Galectins are multi-purpose effectors acting via interactions with distinct counterreceptors based on protein-glycan/protein recognition. We report here the first crystallographic information on the N-terminal extension of the carbohydrate recognition domain of rat galectin-5, which is precisely described as an N-tailed proto-type-like galectin. The overall fold in ligand-free and -loaded rGal-5 is composed of two antiparallel β-sheets (F1 to F5 and S1 to S6 strands) that form the characteristic β-sandwich structure. The presented data shows that the N-terminal extension can adopt an ordered structure and shapes the hypothesis that a ligand-induced shift in the equilibrium between flexible and ordered conformers potentially acts as a molecular switch, enabling new contacts in this region.

Our attempts to crystallize rGal-5 bound to the blood-group B tetrasaccharide were unsuccessful. Thus, we decided to test chicken GRIFIN (cGRIFIN) as a model for the binding of this compound. We were able to obtain crystals of cGRIFIN in the presence of the blood-group B tetrasaccharide. These crystals diffracted up to a resolution of 1.14 Å. The GalB moiety fully superposes with the galactose moiety of lactose, forming H-bonds with His46, Asn48, Arg50, Asn59 and Glu69. On the other hand, the GlcNacB moiety is rotated in the tetrasaccharide compared to the glucose moiety of lactose. The GalA moiety establishes two additional H-bonds, one of them linking the 6′-hydroxyl group with the NE atom of Trp66. The second one extends the binding site beyond the S4 strand, linking the 2′-hydroxyl group with Glu32. The superposition of the lactose-bound rGal-5 structure with the blood-group B tetrasaccharide-bound cGRIFIN gave an RMSD of 0.69 Å for all Cα atoms, showing the similarity of both complexes.

>MALRFEALYPEGMCPGWSVVVKGKTSSNTSMFEINFLSHPGDQIAFHFNPRFASSRIVCNSFLANHWGKEEVNKTFPFEAKEPFQVEIYSDQDYFHIFIDENKILQYKHRQKQLSSITKLQILNDIEISSVEITKRGLY[2x]>[3x]MMKRNILAVIVPALLVAGTANAAEIYNKDGNKVDLYGKAVGLHYFSKGNGENSYGGNGDMTYARLGFKGETQINSDLTGYGQWEYNFQGNNSEGADAQTGNKTRLAFAGLKYADVGSFDYGRNYGVVYDALGYTDMLPEFGGDTAYSDDFFVGRVGGVATYRNSNFFGLVDGLNFAVQYLGKNERDTARRSNGDGVGGSISYEYEGFGIVGAYGAADRTNLQEA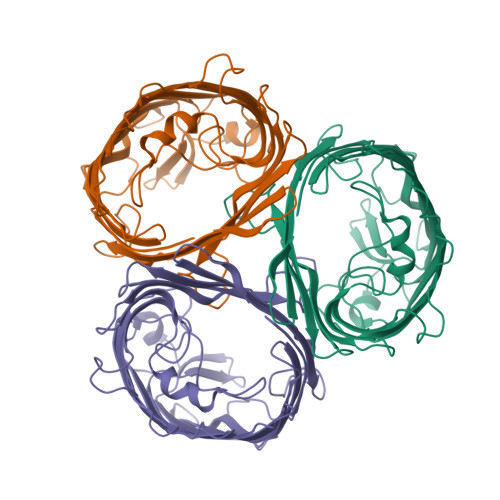QPLGNGKKAEQWATGLKYDANNIYLAANYGETRNATPITNKFTNTSGFANKTQDVLLVAQYQFDFGLRPSIAYTKSKAKDVEGIGDVDLVNYFEVGATYYFNKNMSTYVDYIINQIDSDNKLGVGSDDTVAVGIVYQF>[2x]TKPLDGINVLDFTHVQAGPACTQMMGFLGANVIKIERRGSGDMTRGWLQDKPNVDSLYFTMFNCNKRSIELDMKTPEGKELLEQMIKKADVMVENFGPGALDRMGFTWEYIQELNPRVILASVKGYAEGHANEHLKVYENVAQCSGGAAATTGFWDGPPTVSGAALGDSNSGMHLMIGILAALEIRHKTGRGQKVAVAMQDAVLNLVRIKLRDQQRLERTGILAEYPQAQP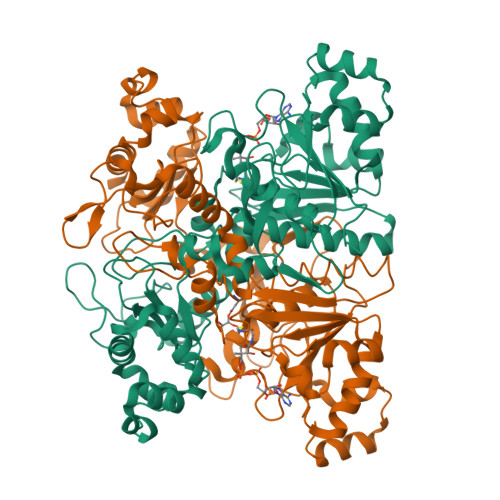NFAFDRDGNPLSFDNITSVPRGGNAGGGGQPGWMLKCKGWETDADSYVYFTIAANMWPQICDMIDKPEWKDDPAYNTFEGRVDKLMDIFSFIETKFADKDKFEVTEWAAQYGIPCGPVMSMKELAHDPSLQKVGTVVEVVDEIRGNHLTVGAPFKFSGFQPEITRAPLLGEHTDEVLKELGLDDAKIKELHAKQVV>[4x]SMASVAEYGGEVSFKYAQSKGEVYKEIVKHVDTQHGVSESTCAHWIANKVSSQGEDFWNTMYEGGKKGHLKQEAIDSIKKLQTEFMQSGSATQQFKLTDNWLQEQGVVPKEKKVG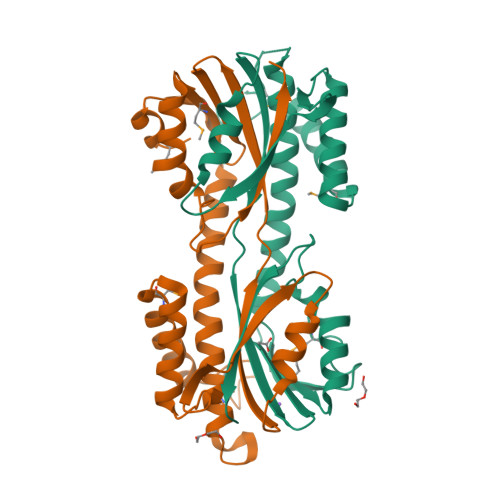DLSRRDEVAGTVSKSDISALTKAILDTGSDTAGAKKISINLEGGSHTVSALVQGEKVVFFDPNFGEMTFPSHQKFESWLKEAFWEKSGYAGKKEGKRFFNVVNYHAE alpha-D-threo-hexo-2,5-diulo-5,1-pyranosyl 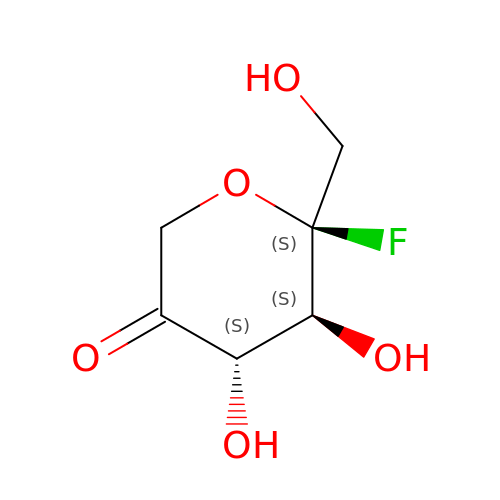fluoride | C6 H9 F O5 | VCJAHEOIRFFLTQ-NGJCXOISSA-N In this work, we have sought to understand the evolutionary history of lipid II targeting glycopeptide antibiotics (GPAs), a vital class of nonribosomal peptides used in the clinic for the treatment of resistant bacterial infections and exemplified by vancomycin (Van) and teicoplanin (Tei). Since ANC1-3 domains display polydisperse elution profiles in size exclusion chromatography, we instead turned to the characterisation of an Acore construct of the Hpg accepting A1 domain from Tei biosynthesis (A1tei), which possesses a homologous pocket to ANC1. The MbtH-like domain Tcp13 also exhibits the anticipated fold, containing a 3-stranded antiparallel β-sheet and an α-helix adjoining the centre of the sheet.

To visualise how the ancestral GPA Hpg pocket evolved to select alternate substrates, we turned to structural methods. The Hpg substrate is coordinated by three H-bonds to the α-amino group, one to the side group of D196 and two to the backbone carbonyl groups of L295 and G289. The aromatic ring of L-Hpg is stabilised by hydrophobic interactions with the sidechain of L295 and the main chain of G264, whilst the phenol moiety of L-Hpg is hydrogen bonded to H237 and to the amide nitrogen of G263. The orientation of the H237 imidazole is maintained through three key interactions, two being hydrophobic interactions between the imidazole C5 and L261/L287. A water mediated interaction between E201 and the imidazole Nπ further contributes to imidazole positioning. This Glu residue is widely conserved among NRPS A-domains and serves to maintain the desired orientation of the loop immediately prior to the key α-amino coordinating acidic residue (D196 in A1tei).

>[2x]MSTVPELLARQVTRAPDAVAVVDRDRVLTYRELDELAGRLSGRLIGRGVRRGDRVAVLLDRSADLVVTLLAIWKAGAAYVPVDAGYPAPRVAFMVADSGASRMVCSAATRDGVPEGIEAIVVTDEEAFEASAAGARPGDLAYVMYTSGSTGIPKGVAVPHRSVAELAGNPGWAVEPGDAVLMHAPYAFDASLFEIWVPLVSGGRVVIAEPGPVDARRLREAISSGVTRAHLTAGSFRAVAEESPESFAGLREVLTGGDVVPAHAVARVRSACPRVRIRHLYGPTETTLCATWHLLEPGDEIGPVLPIGRPLPGRRAQVLDASLRAVAPGVIGDLYLSGAGLADGYLRRAGLTAERFVADPSAPGARMYRTGDLAQWTADGALLFAGRADDQGSHHHHHH;>[2x]MTNPFDNEDGSFLVLVNGEGQHSLWPAFAEVPDGWTGVHGPASRQDCLGYVEQNWTDLRPKSLISQISD2,3-DIHYDROXY-VALERIANIC ACID | C6 H12 O4 | 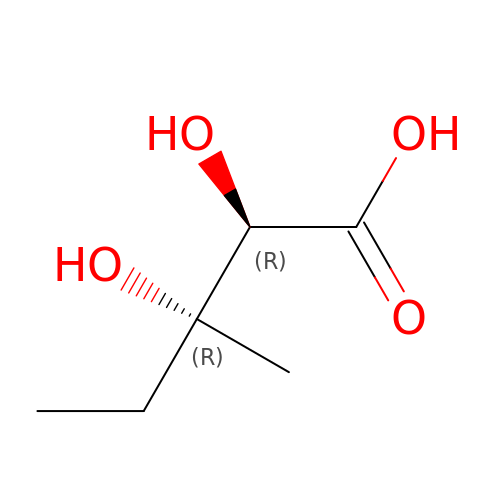PDGXJDXVGMHUIR-UJURSFKZSA-N>LHRNSLIVLADVALFLALYHFLPFEHNVVLGISMLAFIAVLWLTEALHVTVTAILVPVMAVFFGIFETQAALNNFANSIIFLFLGGFALAAAMHHQGLDKVIADKVLAMAQGKMSVAVFMLFGVTALLSMWISNTATAAMMLPLVLGVLSKVDADKQRSTYVFVLLGVAYSASIGGIATLVGSPPNAIAAAEVGLSFTDWMKFGLPTAMMMLPMAIAILYFLLKPTLNGMFELDRAPVNWDKGKVVTLGIFGLTVFLWIFSSPINAALGGFKSFDTLVALGAILMLSFARVVHWKEIQKTADWGVLLLFGGGLCLSNVLKQTGTSVFLANALSDMVSHMGIFVVILVVATFVVFLTEFASNTASAALLIPVFATVAEAFGMSPVLLSVLIAVAASCAFMLPVATPPNAIVFASGHIKQSEMMRVGLYLNIACIGLLTAIAMLFWQ[4x]

Membrane transporters belonging to the ubiquitous divalent anion/Na+ symporter (DASS) family move Krebs cycle intermediates or sulphate across the cell membrane typically by utilizing the preexisting Na+ gradient. However, like other well-characterized bacterial DASS proteins, VcINDY is known to transport succinate and other C4-dicarboxylates, rather than citrate (C6-tricarboxylate)1319. Our structure reveals a homodimeric arrangement, with each VcINDY protomer comprising eleven membrane-spanning helices (TM1–TM11), two re-entrant helix-turn-helix hairpins (HPin and HPout) and two interfacial helices (H4c and H9c). Viewed in parallel to the membrane, the VcINDY dimer is shaped like an inverted bowl with its concave mouth facing the cytoplasm, allowing the aqueous solution to reach the midpoint of the membrane.

Herein we present the structure of succinate-bound VcINDY at a resolution of 2.8 Å, which, to our knowledge, offers the first molecular view of a substrate-bound DASS. We crystallized VcINDY in the presence of succinate and Na+, and determined the structure by combining molecular replacement and multiple isomorphous replacement and anomalous scattering (MIRAS) phasing. Within this cleft, the binding sites of two Na+ ions, designated as Na1 and Na2, were observed. Specifically, Na+ in Na1 is coordinated to the side-chain hydroxyl of S146 and side-chain carbonyl of N151, in addition to the main-chain carbonyls of S146, S150 and G199; whereas Na+ in Na2 binds to the side-chain hydroxyl of T373 and side-chain carbonyl of N378, besides the backbone carbonyls of T373, A376 and A420. Within the Na+-binding cleft in VcINDY, the electron density for succinate was also observed. The bound succinate makes contacts with VcINDY mainly through H-bonding interactions and is partly exposed to cytoplasm, indicating that the transporter adopts an inward-open conformation. Specifically, the side-chain amide of N151 and the side-chain hydroxyl of T152 donate H-bonds to one carboxylate in succinate, whereas the side-chain hydroxyl S377 and the side-chain amide of N378 make contacts with the other succinate carboxylate. Significantly, the bound succinate adopts an extended conformation, structurally mimicking fumarate, a C4-dicarboxylate with a central trans double bond. In the succinate-binding VcINDY, the Na+ ions in Na1 and Na2 coordinate several succinate-binding amino acids and thus stabilize the conformation of these amino-acid side chains. Furthermore, the amino ends of four short helices from HPin, HPout, TM5 and TM10, which possess localized positive dipoles, all point toward the bound succinate and stabilize its two negative charges (crystallization pH∼7).>[6x]DRPSYCNLPADSGSGTKSEQRIYYNSARKQCLTFTYNGKGGNENNFIHTYDCARTCQY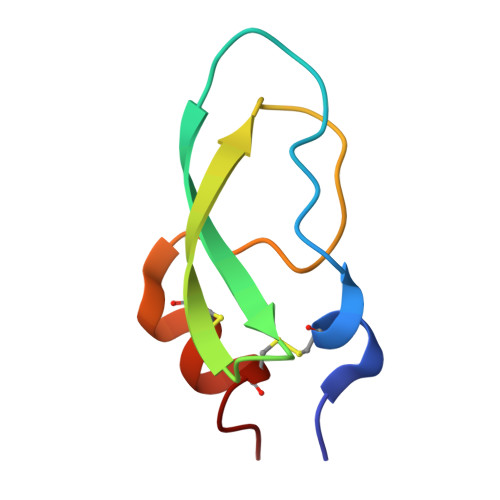PA>[2x]MPNVRNPFDLLLLPTWIVPVEPAGVVLRDHALGIRDGQIALVAPREQAMRHGATEIRELPGMLLAPGLVNAHGHSAMSLFRGLADDLPLMTWLQDHIWPAEGQWVSEDFIRDGTELAIAEQVKGGITCFSDMYFYPQAICGVVHDSGVRAQVAIPVLDFPIPGARDSAEAIRQGMALFDDLKHHPRIRIAFGPHAPYTVSDDKLEQILVLTEELDASIQMHV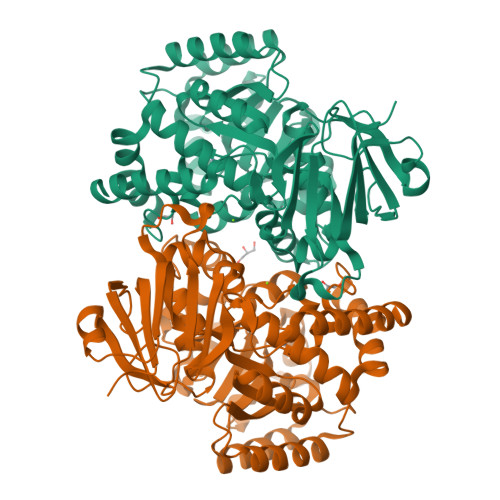HETAFEVEQAMERNGERPLARLHRLGLLGPRFQAVHMTQVDNDDLAMLVETNSSVIHCPESNLKLASGFCPVEKLWQAGVNVAIGTDGAASNNDLDLLGETRTAALLAKAVYGQATALDAHRALRMATLNGARALGLERLIGSLEAGKAADLVAFDLSGLAQQPVYDPVSQLIYASGRDCVRHVWVGGRQLLDDGRLLRHDEQRLIARAREWGAKIAASDRSAENLYFQ> ATCDDGRTTANAACCILFPILDDIQENLFDGAQCGEEVHESLRLTFHDAIGFSPTL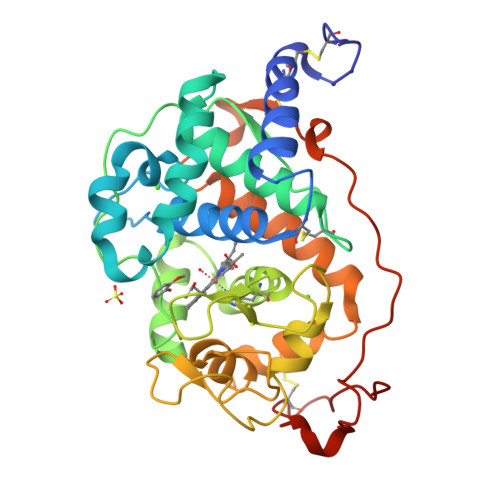GGGGADGSIIAFDTIETNFPANAGIDEIVSAQKPFVAKHNISAGDFIQFAGAVGVSNCPGGVRIPFFLGRPDAVAASPDHLVPGPFDSVDSILARMGDAGFSPVEVVWLLASHSIAAADKVDPSIPGTPFDSTPEVFDSQFFIETQLKGRLFPGTADNKGEAQSPLQGEIRLQSDHLLARDPQTACEWQSMVNNQPKIQNRFAATMSKMALLGQDKTKLIDCSDVIPTPPALVGAAHLPAGFSLSDVEQACAATPFPALTA>[2x]KKMAFTLADRVTEEMLADKAALVVEVVEENYHDAPIVGIAVVNEHGRFFLRPETALADPQFVAWLGDETKKKSMFDSKRAAVALKWKGIELCGVSFDLLLAAYLLDPAQGVDDVAAAAKMKQYEAVRPDEAVYGKGAKRAVPDEPVLAEHLVRKAAAIWE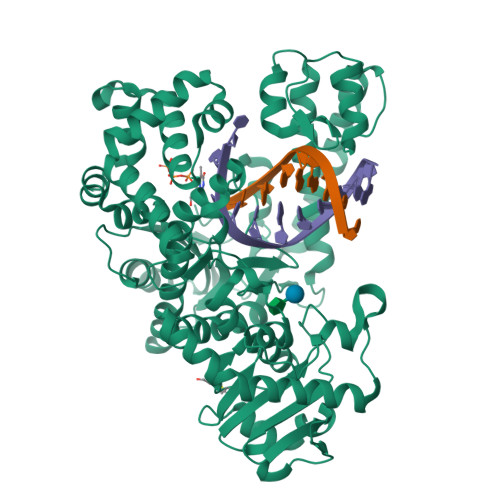LERPFLDELRRNEQDRLLVELEQPLSSILAEMEFAGVKVDTKRLEQMGKELAEQLGTVEQRIYELAGQEFNINSPKQLGVILFEKLQLPVLKKTKTGYSTSADVLEKLAPYHEIVENILHYRQLGKLQSTYIEGLLKVVRPATKKVHTIFNQALTQTGRLSSTEPNLQNIPIRLEEGRKIRQAFVPSESDWLIFAADYSQIELRVLAHIAEDDNLMEAFRRDLDIHTKTAMDIFQVSEDEVTPNMRRQAKAVNYGIVYGISDYGLAQNLNISRKEAAEFIERYFESFPGVKRYMENIVQEAKQKGYVTTLLHRRRYLPDITSRNFNVRSFAERMAMNTPIQGSAADIIKKAMIDLNARLKEERLQAHLLLQVHDELILEAPKEEMERLCRLVPEVMEQAVTLRVPLKVDYHYGSTWYDAK>[4x]HHHHHHNKDLKGLYAALLVPFDENGQVNEQGLKQIAQNAIETEELDGLYVNGSSGENFLLNTEQKKQVFKVAKEAVGDKVKLIAQVGSLDLNEAIELGKYATELGYDALSAVTPFYYPFTFEEIRDYYFDIIEATQNNMIIYAIPDLTGVNISIEQFSELFNHEKIVGVCYTAPNFFLLERIRKAFPDK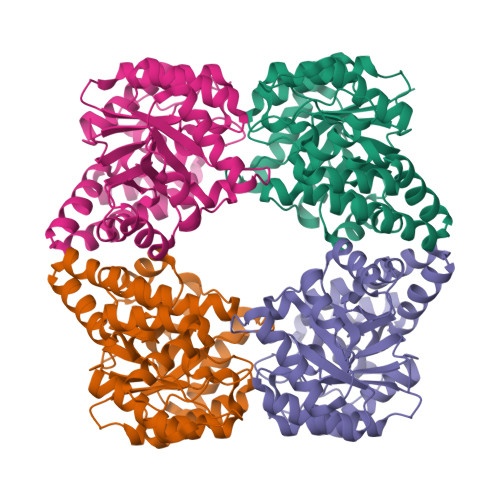LILSGFDEMLVQATISGVDGAIGSTYNVNGRRARKIFDLARQGQIQEAYQLQHDSNDIIETVLSMGIYPTLKEILRHRGIDAGLPKRPFKPFNEAHRQTLDQLIAKYDL> MRQVDAATHGGRAVIELREKILSGELPGGMRLFEVSTAELLDISRTPVREALSRLTEEGLLNRLPGG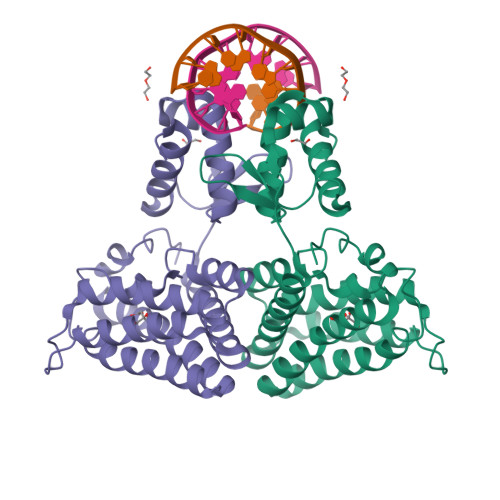GFVVRRFGFADVVDAIEVRGVMEGTAARLAAERGVSKVALEEIDATVQQLDLCFGDRVDDVDFDGYAALNRIFHHQLAALCGSEMIRREVERASSLPFASPSAFLPDKANIGAFRRSLRGAQEQHKAIVAAIVAREGARAEAVAREHSRTARTNLEYMIREAPELIAQVPGLALISDHHHHHH>MASSVGNVADSTEPTKRMLSFQGPMELAHREYQAGDFEAAERHCMQLWRQEPDNTGVLLLLSSIHFECRRLDRSAHFSTLAIKQNPLLAEAYSNLGNVYKERGQLQEAIEHYRHALRLKPDFIDGYINLAAALVAAGDMEGAVQAYVSALQYNPDLYCVRSDLGNLLKALGRLEEAKACYLKAIETQPNFAVAWSNLGCVFNAQGEIWLAIHHFEKAVTLDPNFLDAYINLGNVLKEARIFDRAVAAYLRALSLSPNHAVVHGNLACVYYEQGLIDLAIDTYRRAIELQPHFPDAYCNLANALKEKGSVAEAEDCYNTALRLCPTHADSLNNLANIKREQGNIEEAVRLYRKALEVFPEFAAAHSNLASVLQQQGKLQEALMHYKEAIRISPTFADAYSNMGNTLKEMQDVQGALQCYTRAIQINPAFADAHSNLASIHKDSGNIPEAIASYRTALKLKPDFPDAYCNLAHCLQIVCDWTDYDERMKKLVSIVADQLEKNRLPSVHPHHSMLYPLSHGFRKAIAERHGNLCLDKINVLHKPPYEHPKDLKLSDGRLRVGYVSSDFGNHPTSHLMQSIPGMHNPDKFEVFCYALSPDDGTNFRVKVMAEANHFIDLSQIPCNGKAADRIHQDGIHILVNMNGYTKGARNELFALRPAPIQAMWLGYPGTSGALFMDYI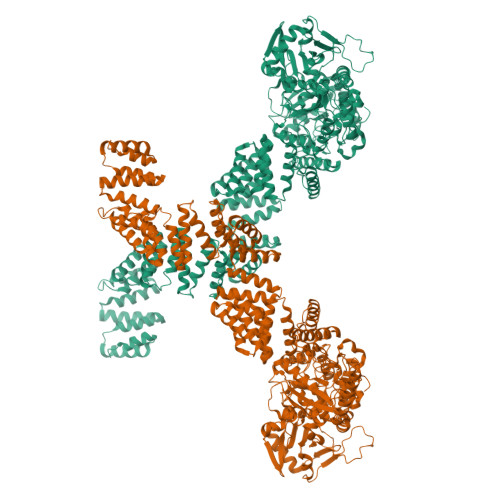ITDQETSPAEVAEQYSEKLAYMPHTFFIGDHANMFPHLKKKAVIDFKSNGHIYDNRIVLNGIDLKAFLDSLPDVKIVKMKCPDGGDNADSSNTALNMPVIPMNTIAEAVIEMINRGQIQITINGFSISNGLATTQINNKAATGEEVPRTIIVTTRSQYGLPEDAIVYCNFNQLYKIDPSTLQMWANILKRVPNSVLWLLRFPAVGEPNIQQYAQNMGLPQNRIIFSPVAPKEEHVRRGQLADVCLDTPLCNGHTTGMDVLWAGTPMVTMPGETLASRVAASQLTCLGCLELIAKNRQEYEDIAVKLGTDLEYLKKVRGKVWKQRISSPLFNTKQYTMELERLYLQMWEHYAAGNKPDHMIKPVEVTESAHHHHHH[2x]>GCGATATACGU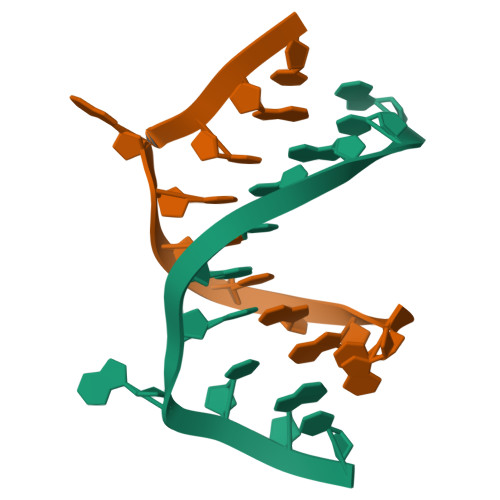[6x]>MKHTLPDLPFDYADLEPVISHEIMQLHHQKNHATYVNNLNQIEEKLHEAVSKGNLKEAIALQPALKFNGGGHINHSIFWTNLAKDGGEPSKELMDTIKRDFGSLDNLQKRLSDITIAVQGSGWGWLGYCKKDKILKIATCANQDPLEGMVPLFGIDVWEHAYYLQYKNVRPDYVHAIWKIANWK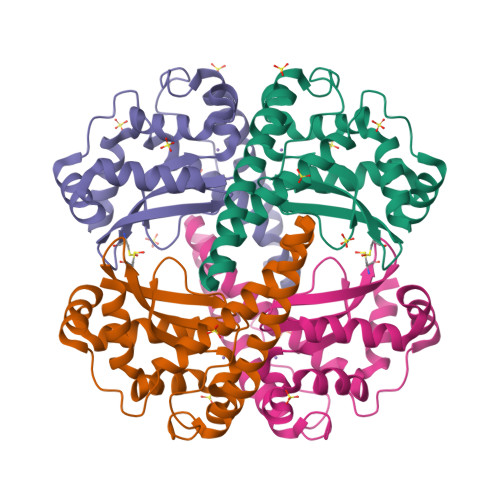NISERFANARQ[2x]>[4x]MDAKARNCLLQHREALEKDIKTSYIMDHMISDGFLTISEEEKVRNEPTQQQRAAMLIKMILKKDNDSYVSFYNALLHEGYKDLAALLHDGIPVVSSSSGKDSVSGITSYVRTVLCEGGVPQRPVVFVTRKKLVNAIQQKLSKLKGEPGWVTIHGMAGCGKSVLAAEAVRDHSLLEGCFPGG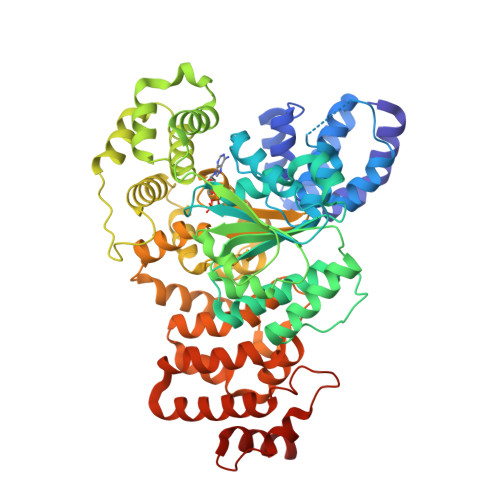VHWVSVGKQDKSGLLMKLQNLCTRLDQDESFSQRLPLNIEEAKDRLRILMLRKHPRSLLILDDVWDSWVLKAFDSQCQILLTTRDKSVTDSVMGPKYVVPVESSLGKEKGLEILSLFVNMKKADLPEQAHSIIKECKGSPLVVSLIGALLRDFPNRWEYYLKQLQNKQFKRIRKSSSYDYEALDEAMSISVEMLREDIKDYYTDLSILQKDVKVPTKVLCILWDMETEEVEDILQEFVNKSLLFCDRNGKSFRYYLHDLQVDFLTEKNCSQLQDLHKKIITQFQRYHQPHTLSPDQEDCMYWYNFLAYHMASAKMHKELCALMFSLDWIKAKTELVGPAHLIHEFVEYRHILDEKDCAVSENFQEFLSLNGHLLGRQPFPNIVQLGLCEPETSEVYQQAKLQAKQEVDNG> EALANGTVMSGSHWGVFTATVENGRATAFTPWEKDPHPTPMLEGVLDSIYSPTRIKYPMVRREFLEKGVNADRSTRGNGDFVRVSWDQALDLVAAEVKRVEETYGPQGVFGGSYGWKSPGRLHNCTTLLRRMLTLAGGYVNGAGDYSTGAAQVIMPHVVGTLEVYEQQTAWPVLAENTEVMVFWAADPIKTSQIGWVIPEHGAYPGLEALKAKGTKVIVIDPVRTKTVEFFGADHVTPKPQTDVAIMLGMAHTLVAEDLYDKDFIANYTSGFDKFLPYLMGETDSTPKTAEWASDISGVPAETIKELARLFKSKRTMLAAGWSMQRMHHGEQAHWMLVTLASMLGQIGLPGGGFGLSYHYSGGGTPSSSGPALSGITDGGAATKGPEWLAASGASVIPVARVVDMLENPGAEFDFNGTRSKFPDVKMAYWVGGNPFVHHQDRNRMVKAWEKLETFIVHDFQWTPTARHADIVLPATTSYERNDIETIGDYSNTGILAMKKIVEPLYEARSDYDIFAAVAERLGKGKEFTEGKDEMGWIKSFYDDAAKQGKAGGVEMPAFDAFWAEGIVEFPVTDGADFVRYASFREDPLLNPLGTPTGLIEIYSKNIEKMGYDDCPAHPTWMEPLERLDGPGAKYPLHIAASHPFNRLHSQLNGTVLREGYAVQGHEPCLMH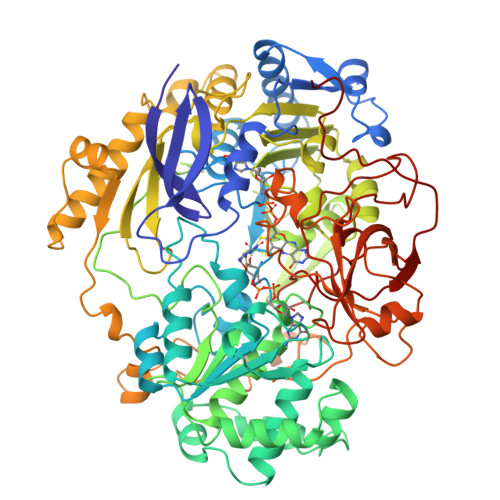PDDAAARGIADGDVVRVHNDRGQILTGVKVTDAVMKGVIQIYEGGWYDPSDVTEAGTLDKYGDVNVLSADIGTSKLAQGNCGQTVLAEVEKYTGPAVTLTGFVAPKAAE> VTLTLALAVAFGIAAISPLLARTMGRDAGWPLAAMLGGLALYIWFAIPVDTVASVEWMPALGVELRLSLDPLARVFTMIVLGIGAVVMAYSSRYLGRGSGHGGYYGLMTLFAASMLGLVLADDVVVLFVAWEFTTLCSFFLITLAGPKGTQPAVRTLLVTVAGGLCLLTAAALMVVRTGTTVLSEILVDPVWSADPAFAAVIAVLIAMAAFTKSAQFPFQAWLPDAMVAATPVSAYLHAAAMVKAGIYLLLRFSEALHDVPVWNLLLITCGMTTAVLGAVFAMQRDDLKELLAYSTISQLGFLVATIGVGTPAAMVAAIIHTIAHALFKSSLFMFVGVVDHQTGTRAMSGLPRLYRIMPGTAIGVGLAAASMAGLPPLLGFVSKEWMFKSMLDAPGGAWAGPALGALAVFAATFTFAYSARFLLGGFVTHGPPAGPGPEPVHSTPETIEAPRASFF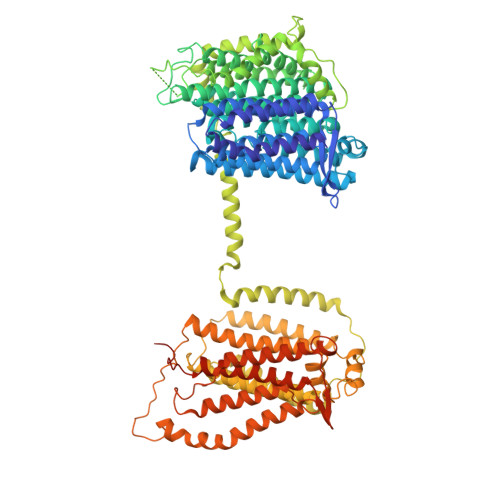LPAALPAVLGLVLGLTGFLLEPAVAAAARASIGEGYEADFGLWHGFAPELFMSMIVITLGIVLVVVRHPVDRFLDRELAPITGVATVDALRRWAIAGGARVGDVTRTDRISRHVWAVLLVLVALAAVGVVAVRPEPEVGSPVRAEDWIVVVLLVVGTAAMVISRSRLGAVANVGIVGFAMALWFFTLGAVDVALTQLLVEVLTVVVIVLVLQRLPRAFHTVSRSRTLVSAAVAIVVGLASGAAVWAMTGRRELSDVGRYFLDNAEQDTGGINVVNTVLVDYRALDTLGELTVLGVAGLAVILALHARRALPRRDVPLAVHADSPLLSAQDNGVFLRTFARILGPLIVLLSLYFLVRGHNAPGGGFNSALIGGAGIAIYYLRAPSDKAARIRVPYVAVIAAGVIIGVVTGLAGFVDGSFLLPLHAYLGDVHLTTALIFDVGVYLAVLGVIMAAIDKLGGDDRSDEPAVPPPPPTGPGAEATAPAATEDADRVIDVTDNREVQA>[2x]MAAEGYGAASPATATTQDGAKGAAPPNPAASINSPAPAANPEKLTPAQLKAKAKAEKQARRAAAKEAKSAVAAAGQPAQQSGSAGADSKGAAKGKGKQEGQQVPPKGVLVHRPSVSGRRPSIMVVEKDARSGIPECFSHIPMAKRIPTSQAHKDVHPAVLAVGQQMATFALKDSISRLKATLLAFRKVIESYETPKGNSLSRHFVPHVLNPQIEYLTECRPMCFAM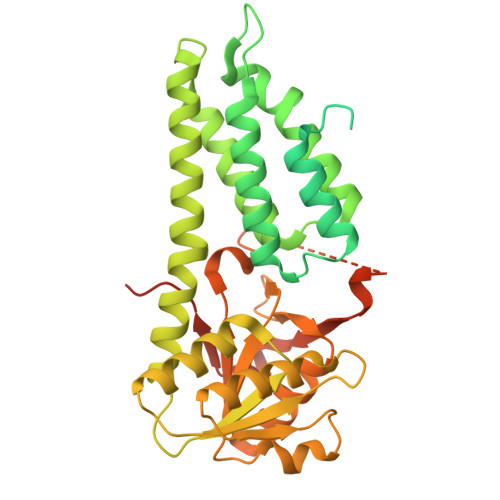GNAIRLLKAKVNKFDINTPEDEAKEGLLEWIDFLINERITLAEYVIARNAAQSINDGDTIVTYGRHRLVEKTLLRARKEGKSFNVTVLDDPYVGEGKELAKVLRHAGIPVLYSPNLGGLRSKVPAASNVFLGGEAIFANGSLHAPSGTADVAMAATNAGAKVIVLCETINFDRERVSVDALTYNEIDPERNTGDCFRLLFDNTHERYITGVITEIEFGGGNSPAQAILALLRKQEDPLIA5-N-ALLYL-ARGININE | C9 H19 N4 O2 | 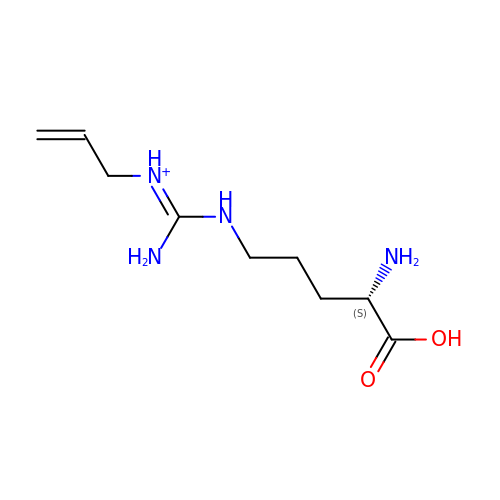ZPQWZDPOLXVMOU-ZETCQYMHSA-O> HHHHHHPEIVDTCSLASPASVCRTKHLHLRCSVDFTRRTLTGTAALTVQSQEDNLRSLVLDTKDLTIEKVVINGQEVKYALGERQSYKGSPMEISLPIALSKNQEIVIEISFETSPKSSALQWLTPEQTSGKEHPYLFSQCQAIHCRAILPCQDTPSVKLTYTAEVSVPKELVALMSAIRDGETPDPEDPSRKIYKFIQKVPIPCYLIALVVGALESRQIGPRTLVWSEKEQVEKSAYEFSETESMLKIAEDLGGPYVWGQYDLLVLPPSFPYGGMENPCLTFVTPTLLAGDKSLSNVIAHQISHSWTGNL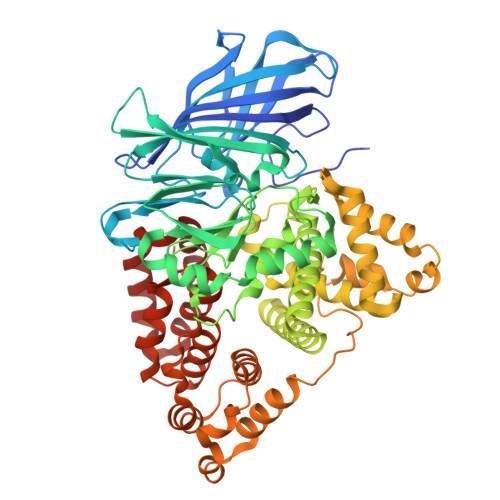VTNKTWDHFWLNEGHTVYLERHICGRLFGEKFRHFNALGGWGELQNSVKTFGETHPFTKLVVDLTDIDPDVAYSSVPYEKGFALLFYLEQLLGGPEIFLGFLKAYVEKFSYKSITTDDWKDFLYSYFKDKVDVLNQVDWNAWLYSPGLPPIKPNYDMTLTNACIALSQRWITAKEDDLNSFNATDLKDLSSHQLNEFLAQTLQRAPLPLGHIKRMQEVYNFNAINNSEIRFRWLRLCIQSKWEDAIPLALKMATEQGRMKFTRPLFKDLAAFDKSHDQAVRTYQEHKASMHPVTAMLVGKDLKVD> AT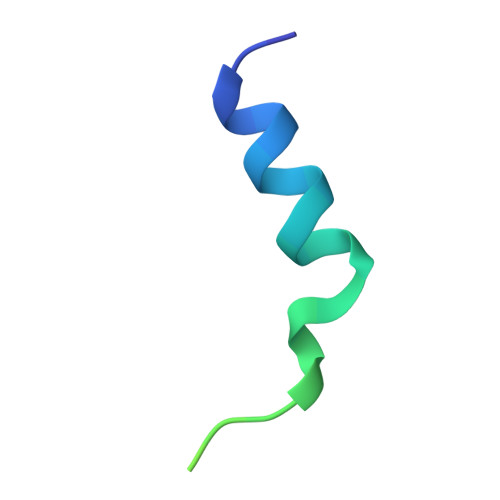FWERVRSILKSGLNFASTIPGPVGVAATGIKGIIETIGSLWV(2~{S})-2-[2-[3-[[(2~{R})-4-[[[(2~{R},3~{S},4~{R},5~{R})-5-(6-aminopurin-9-yl)-4-oxidanyl-3-phosphonooxy-oxolan-2-yl]methoxy-oxidanyl-phosphoryl]oxy-oxidanyl-phosphoryl]oxy-3,3-dimethyl-2-oxidanyl-butanoyl]amino]propanoylamino]ethylsulfanyl]propanoic 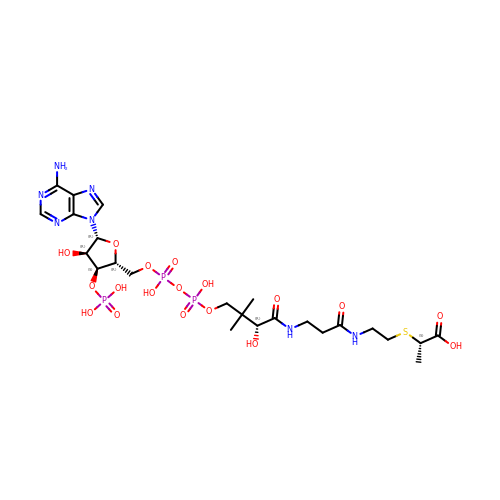acid | C24 H40 N7 O18 P3 S | ULCSPOREAVNZTJ-IBNUZSNCSA-N> MIAGTPPHSTMERGGDRDIVVTGARNQFAPDLEPGGSVSCMRSSLSFLSLIFDVGPRDVLSAEAIEGCLVEGGEWTRATAGPGPPRMCSIVELPNFLEYPGARGGLRCVFSRVYGEVGFFGEPAAGLLETQCPAHTFFAGPWALRPLSYTLLTIGPLGMGLFRDGDTAYLFDPHGLPEGTPAFIAKVRAGDMYPYLTYYTRDRPDVRWAGAMVFFVPSGPEPAAPADLTAAALHLYGASETYLQDEAFSERRVAITHPLRGEIAGLGEPCVGVGPREGVGGPGPHPPTAAQSPPPTRARRDDRASETSRGTAGPSAKPEAKRPNRAPDDVWAVALKGTPPTDPPSADPPSADPPSAIPPPPPSAPKTPAAEAAEEDDDDMRVLEMGVVPVGRHRARYSAGLPKRRRPTWTPPSSVEDLTSGEKTKRSAPPAKTKKKSTPKGKTPVGAAVPASVPEPVLASAPPDPAGPPVAEAGEDDGPTVPASSQALEALKTRRSPEPPGADLAQLFEAHPNVAATAVKFTACSAALAREVAACSRLTISALRSPYPASPGLLELCVIFFFERVLAFLIENGARTHTQAGVAGPAAALLEFTLNMLPWKTAVGDFLASTRLSLADVAAHLPLVQHVLDENSLIGRLALAKLILVARDVIRETDAFYGELADLELQLRAAPPANLYTRLGEWLLERSQAHPDTLFAPATPTHPEPLLYRVQALAKFARGEEIRVEAEDRQMREALDALARGVDAVSQHAGPLGVMPAPAGAAPQGAPRPPPLGPEAVQVRLEEVRTQARRAIEGAVKEYFYRGAVYSAKALQASDNNDRRFHVASAAVVPVVQLLESLPVFDQHTRDIAQRAAIPAPPPIATSPTAILLRDLIQRGQTLDAPEDLAAWLSVLTDAANQGLIERKPLDELARSIRDINDQQARRSSGLAELRRFDALDAALGQQLDSDAAFVPAPGASPYPDDGGLSPEATRMAEEALRQARAMDAAKLTAELAPDARARLRERARSLEAMLEGARERAKVARDAREKFLHKLQGVLRPLPDFVGLKACPAVLATLRASLPAGWSDLPEAVRGAPPEVTAALRADMWGLLGQYRDALEHPTPDTATALSGLHPSFVVVLKNLFADAPETPFLLQFFADHAPIIAHAVSNAINAGSAAVATADPASTVDAAVRAHRVLVDAVTALGAAASDPASPLAFLAAMADSAAGYVKATRLALDARVAIAQLTTLGSAAADLVVQVRRAANQPEGEHASLIQAATRATTGARESLAGHEGRFGGLLHAEGTAGDHSPSGRALQELGKVIGATRRRADELEAATADLREKMAAQRARSSHERWAADVEAVLDRVESGAEFDVVELRRLQALAGTHGYNPRDFRKRAEQALGTNAKAVTLALETALAFNPYTPENQRHPMLPPLAAIHRIDWSAAFGAAADTYADMFRVDTEPLARLLRLAGGLLERAQANDGFIDYHEAVLHLSEDLGGVPALRQYVPFFQKGYAEYVDIRDRLDALRADARRAIGSVALDLAAAAEEISAVRNDPAAAAELVRAGVTLPCPSEDALVACVAALERVDQSPVKDTAYADYVAFVTRQDLADTKDAVVRAKQQRAEATERVTAGLREVLAARERRAQLEAEGLANLKTLLKVVAVPATVAKTLDQARSAEEIADQVEILVDQTEKARELDVQAVAWLEHAQRTFETHPLSAASGDGPGLLTRQGARLQALFDTRRRVEALRRSLEEAEAEWDEVWGRFGRVRGGAWKSPEGFRAACEQLRALQDTTNTVSGLRAQRDYERLPAKYQGVLGAKSAERAGAVEELGGRVAQHADLSARLRDEVVPRVAWEMNFDTLGGLLAEFDAVAGDLAPWAVEEFRGARELIQRRMGLYSAYAKATGQTGAGAAAAPAPLLVDLRALDARARASAPPGQEADPQMLRRRGEAYLRVSGGPGPLVLREATSTLDRPFAPSFLVPDGTPLQYALCFPAVTDKLGALLMCPEAACIRPPLPTDTLESASTVTAMYVLTVINRLQLALSDAQAANFQLFGRFVRHRQARWGASMDAAAELYVALVATTLTREFGCRWAQLEWGGDAAAPGPPLGPQSSTRHRVSFNENDVLVALVASSPEHIYTFWRLDLVRQHEYMHLTLPRAFQNAADSMLFVQRLTPHPDARIRVLPAFSAGGPPTRGLMFGTRLADWRRGKLSETDPLAPWRSVPELGTERGAALGKLSPAQALAAVSVLGRMCLPSTALVALWTCMFPDDYTEYDSFDALLTARLESGQTLSPSGGREASPPAPPNALYRPTGQHVAVPAAATHRTPAARVTAMDLVLAAVLLGAPVVVALRNTTAFSRESELELCLTLFDSRARGPDAALRDAVSSDIETWAVRLLHADLNPIENACLAAQLPRLSALIAERPLARGPPCLVLVDISMTPVAVLWENPDPPGPPDVRFVGSEATEELPFVAGGEDVLAASATDEDPFLARAILGRPFDASLLSGELFPGHPVYQRAPDDQSPSVPNPTPGPVDLVGAEGSLGPGSLAPTLFTDATPGEPVPPRMWAWIHGLEELASDDSGGPAPLLAPDPLSPTADQSVPTSQCAPRPPGPAVTAREARPGVPAESTRPAPVGPRDDFRRLPSPQSSPAPPDATAPRPPASSRASAASSSGSRARRHRRARSLARATQASATTQGWRPPALPDTVAPVTDFARPPAPPKPPEPAPHALVSGVPLPLGPQAAGQASPALPIDPVPPPVATGTVLPGGENRRPPLTSGPAPTPPRVPVGGPQRRLTRPAVASLSESRESLPSPWDP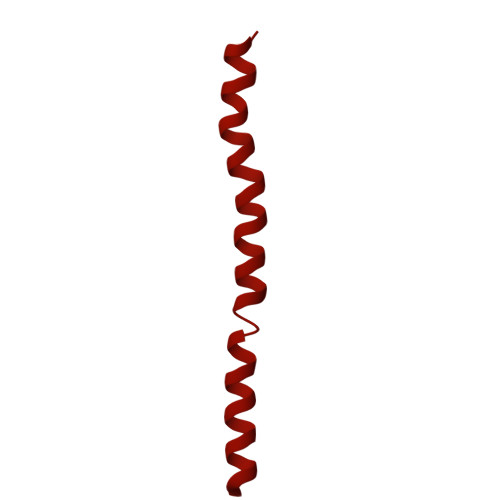ADPTAPVLGRNPAEPTSSSPAGPSPPPPAVQPVAPPPTSGPPPTYLTLEGGVAPGGPVSRRPTTRQPVATPTTSARPRGHLTVSRLSAPQPQPQPQPQPQPQPQPQPQPQPQPQPQPQPQPQPQPQPQPQPQPQPQPQPQPQPQPQPQPQPQPQPQPQNGHVAPGEYPAVRFRAPQNRPSVPASASSTNPRTGSSLSGVSSWASSLALHIDATPPPVSLLQTLYVSDDEDSDATSLFLSDSEAEALDPLPGEPHSPITNEPFSALSADDSQEVTRLQFGPPPVSANAVLSRRYVQRTGRSALAVLIRACYRLQQQLQRTRRALLHHSDAVLTSLHHVRMLLG>MGESERSEAFGIPRDSPLSSGDAAELEQLRREAAVLREQLENAVGSHAPTRSARDIHQLEARIDSLAARNSKLMETLKEARQQLLALREEVDRLGQPPSGYGVLLATHDDDTVDVFTSGRKMRLTCSPNIDAASLKKGQTVRLNEALTVVEAGTFEAVGEISTLREILADGHRALVVGHADEERVVWLADPLIAEDLPDGLPEALNDDTRPRKLRPGDSLLVDTKAGYAFERIPL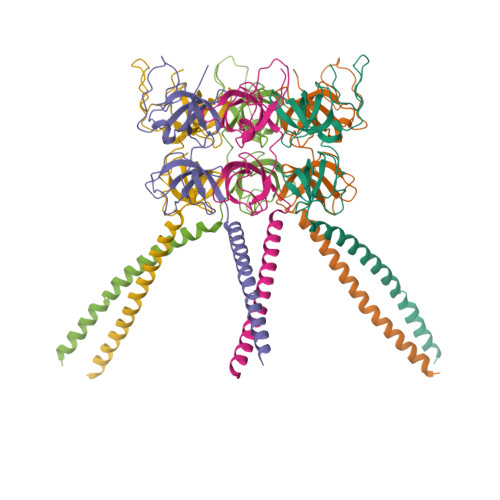VPRGSAAALEHHHHHH[12x]N-(5-methyl-1,2-oxazol-3-yl)acetamide | C6 H8 N2 O2 | 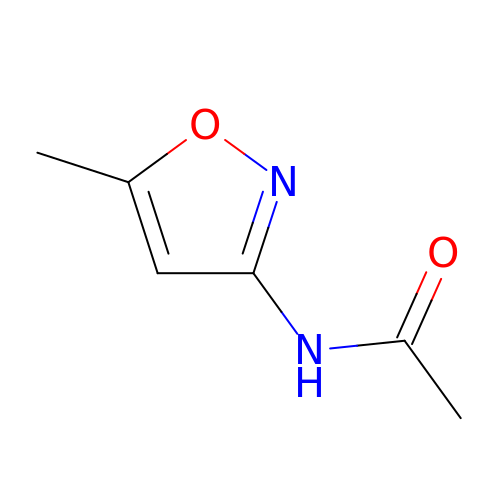CUYZUESBPHQWRI-UHFFFAOYSA-N> SILPEEWLPVLEEGEVHFVRIGELIDRMMEENAGKVKREGETEVLEVSGLEVPSFNRRTNKAELKRVKALIRHDYSGKVYTIRLKSGRRIKITSGHSLFSVRNGELVEVTGDELKPGDLVAVPRRLELPERNHVLNLVELLLGTPEEETLDIVMTIPVKGKKNFFKGMLRTLRWIFGEEKRPRTARRYLRHLEDLGYVRLKKIGYEVLDWDSLKNYRRLYEALVENVRY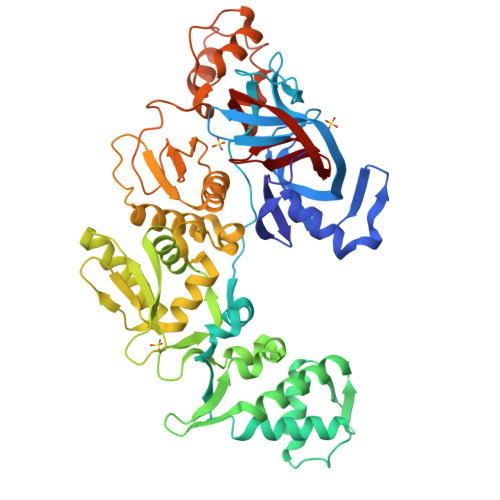NGNKREYLVEFNSIRDAVGIMPLKELKEWKIGTLNGFRMRKLIEVDESLAKLLGYYVSEGYARKQRNPKNGWSYSVKLYNEDPEVLDDMERLASRFFGKVRRGRNYVEIPKKIGYLLFENMCGVLAENKRIPEFVFTSPKGVRLAFLEGYFIGDGDVHPNKRLRLSTKSELLANQLVLLLNSVGVSAVKLGHDSGVYRVYINEELPFVKLDKKKNAYYSHVIPKEVLSEVFGKVFQKNVSPQTFRKMVEDGRLDPEKAQRLSWLIEGDVVLDRVESVDVEDYDGYVYDLSVEDNENFLVGFGLVYAHN>[7x]SNAKAEGKHEWNKNKFLNIAHRGASGHAPEHTFASYDLVKKMKADYLE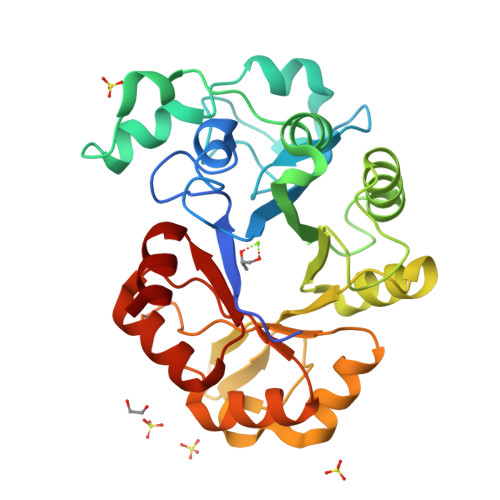LDIQLTKDGQLIAMHDTAVDRTTNGTGEVRDKTLSEIKSLDAGSWFNKAYPEKAKQEYVGQKVPTLEEIFQKYGRSMKYYIETKSPDVYPGMEEKLLALLEKYNLIGQNMSSSRVMIQSFSKDSLKKIHSINKNIPLVQLLWYYPNENNEIVEWSGITHEPKRVTNDDFQEIKKYAVGIGPNLRNDNGDLIINESYMKMARQNGLLIHPYTINEKPDMRLLMKWGATGMFTNYPDRLHTVLKEK>SNAPLADTRFLQRRRALSAQLAAKRIDAMLVTHLTHIRYLSGFTGSNAALIINKDLSARISTDGRYITQIAEQVPDIESLMARNCAPALLSDINGPKRVGFEADYLSVSQCEELRKSAGSDVELIPVT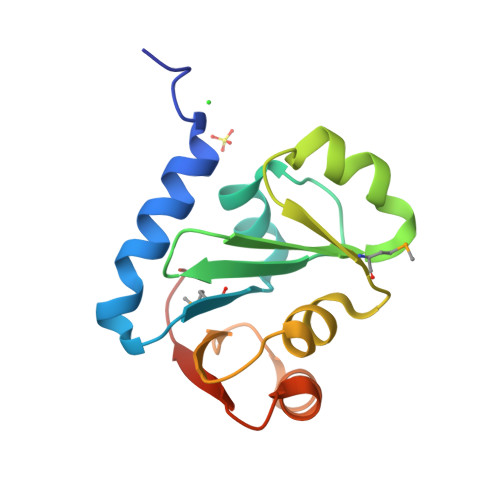GAIEKLR[4x]>[60x]GTGSIGGGKGSGVGISTGGWVGGSHFSDKYVVTKNTRQFITTIQNGHLYKTEAIETTNQSGKSQRCVTTPWTYFNFNQYSCHFSPQDWQRLTNEYKRFRPKAMQVKIYNLQIKQILSNGADTTYNNDLTAGVHIFCDGEHAYPNASHPWDEDVMPDLPYKTWKLFQYGYIPIENELADLDGNAAGGNATEKALLYQMPFFLLENSDHQVLRTGESTEFTFNFDCEWVNNERAYIPPGLMFNPKVPTRRVQYIRQNGSTAASTGRIQPYSKPTSWMTGPGLLSAQRVGPQSSDTAPFMVCTNPEGTHINTGAAGFGSGFDPPSGCLAPTNLEYKLQWYQTPEGTGNNGNIIANPS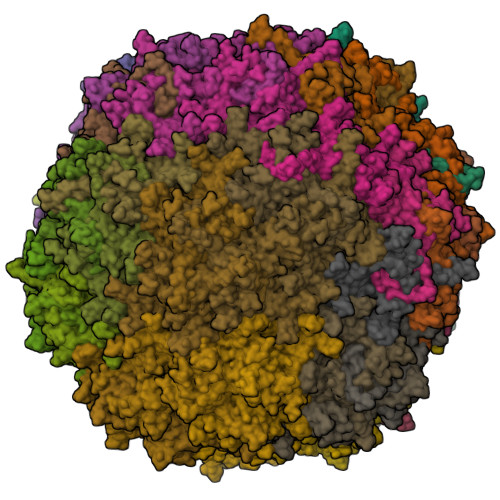LSMLRDQLLYKGNQTTYNLVGDIWMFPNQVWDRFPITRENPIWCKKPRADKHTIMDPFDGSIAMDHPPGTIFIKMAKIPVPTASNADSYLNIYCTGQVSCEIVWEVERYATKNWRPERRHTALGMSLGGESNYTPTYHVDPTGAYIQPTSYDQCMPVKTNINKVL>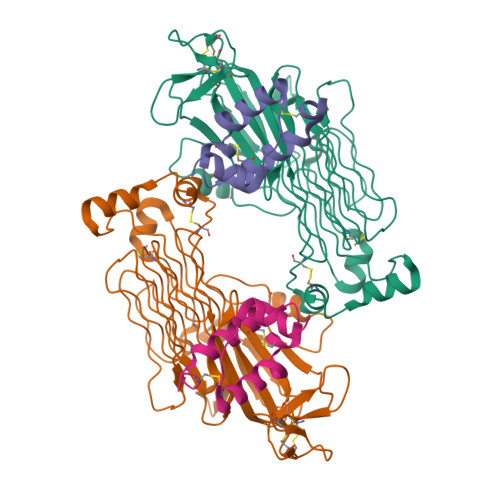GTAPKSRNLFERNPNKELKPGENSPRQTPIFDPTVHWLFTTCGASGPHGPTQAQCNNAYQNSNLSVEVGSEGPLKGIQIWKVPATDTYSISGYGAAGGKGGKNTMMRSHGVSVLGIFNLEKDDMLYILVGQQGEDACPSTNQLIQKVCIGENNVIEEEIRVNRSVHEWAGGGGGGGGATYVFKMKDGVPVPLIIAAGGGGRAYGAKTDTFHPERLENNSSVLGLNGNSGAAGGGGGWNDNTSLLWAGKSLQEGATGGHSCPQAMKKWGWETRGGFGGGGGGCSSGGGGGGYIGGNAASNNDPEMDGEDGVSFISPLGILYTPALKVMEGHGEVNIKHYLNCSHCEVDECHMDPESHKVICFCDHGTVLAEDGVSCIVSP[2x];>[2x]GAEPREPADGQALLRLVVELVQELRKHHSAEHKGLQLLGRDYALGRAEAAGLGPSPEQRVEIVPRDLRMKDKFLKHLTGPLYFSPKCSKHFHRLYHNTRDCTIPAYYKRCARLLTRLAVSPVCMEDKQ> GSMDYKDDDDKKTNWLKRIYRVRPCVKCKVAPRNWKVKNKHLRIYNMCKTCFNNSIDIGDDTYHGHDDWLMYADSKE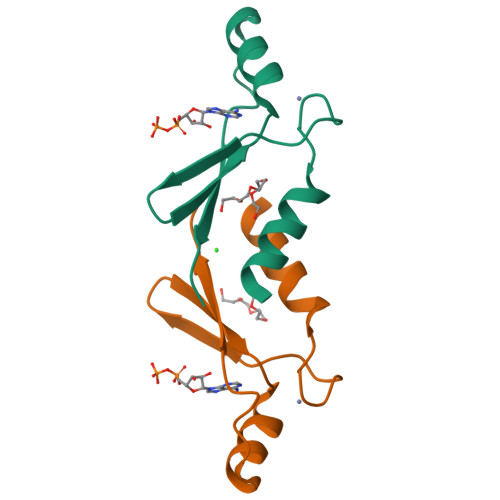ISNT>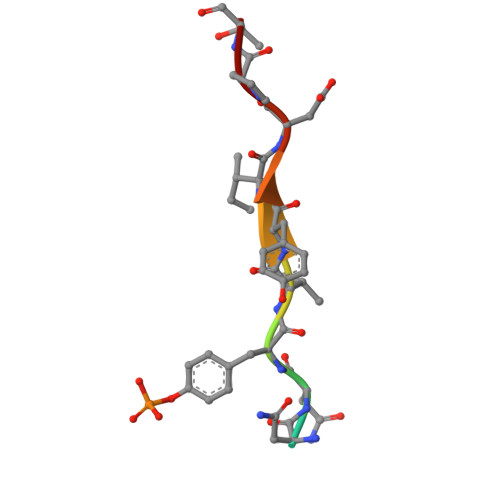 NGNNYVYIDPT> MASNFAAIKAKARRDVHASLSVPARYENYSQDVIVEDLSVRWHNKIAIMGDLENGGYANIVEGIERIIFTREELAVKGVVLSEGDSIIMTAEGYENARLVLKTQEP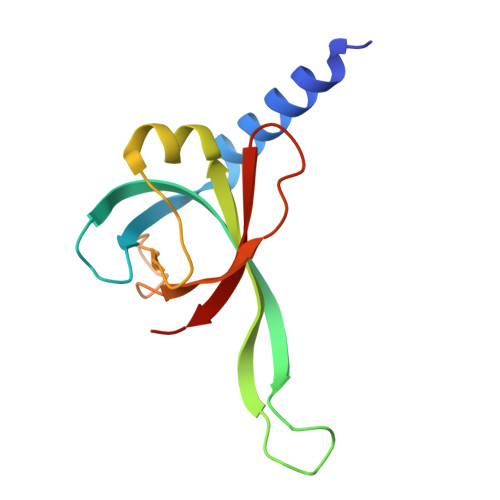IVGPVEVVWQVARAD>[2x]MHPAGIILTKVGYYTIPSMDDLAKITNEKGECIV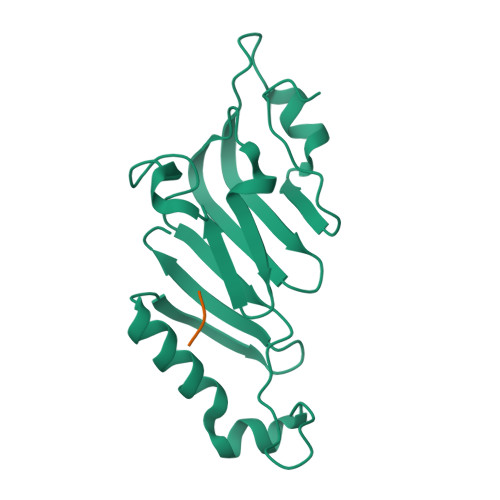SDFTIGRKGYGSIYFEGDVNLTNLNLDDIVHIRRKEVVVYLDDNQKPPVGEGLNRKAEVTLDGVWPTDKTSRCLIKSPDRLADINYEGRLEAVSRKQGAQFKEYRPETGSWVFKVSHF;>[2x]SKYGLQD>[2x]AMGPQEYTLLKLKVLEPYPSKLSGLKGKNIFLVAATLRPETMFGQTNCWVRPDMKYIGFETVNGDIFICTQKAARNMSYQGFTKDNGVVPVVKELMGEEILGASLSAPLTSYKVIYVLPMLTIKEDKGTGVVTSVPSDSPDDIAALRDLKKKQALRAKYGIRDDMVLPFEPVPVIEIPGFGNLSAVTICDELKIQSQNDREKLAEAKEKIYLKGFYEGIMLVDGF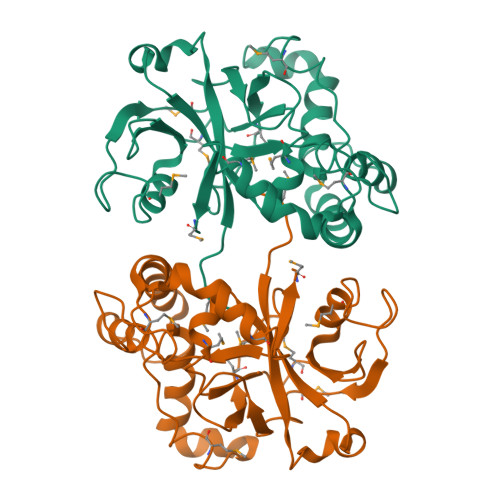KGQKVQDVKKTIQKKMIDAGDALIYME> SSLYKTFFKRNAVFVGTIFAGAFVFQTVFDTAITSWY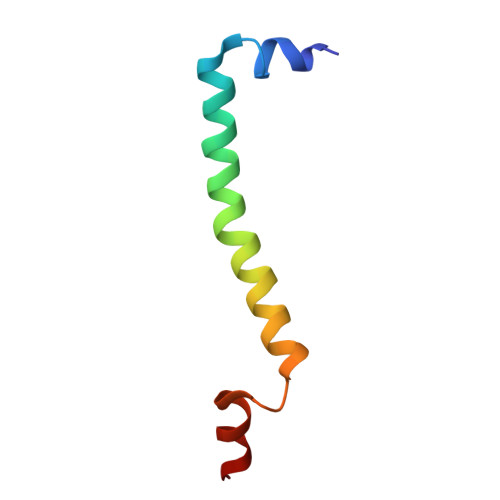ENHNKGKLWKDVKARIA> CUCUCUAAAUAGCAAUAUUUACCUUUGGAGGGAAAAGUUAUCAGGCAUGCACCUGGUAGCUAGUCUUUAAACCAAUAGAUUGCAUCGGUUUAAAAGGCAAGACCGUC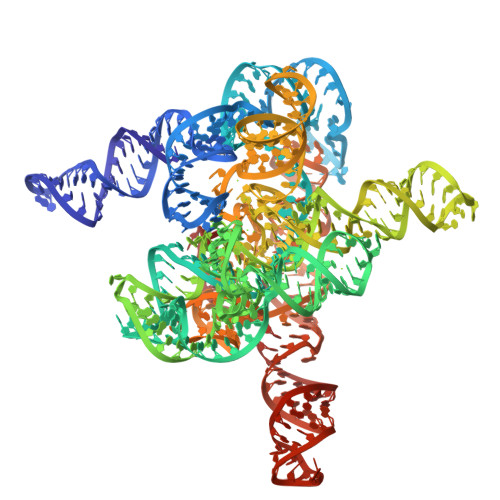AAAUUGCGGGAAAGGGGUCAACAGCCGUUCAGUACCAAGUCUCAGGGGAAACUUUGAGAUGGCCUUGCAAAGGGUAUGGUAAUAAGCUGACGGACAUGGUCCUAACCACGCAGCCAAGUCCUAAGUCAACAGAUCUUCUGUUGAUAUGGAUGCAGUUCACAAACUAAAUGUCGGUCGGGGAAGAUGUAUUCUUCUCAUAAGAUAUAGUCGGACCUCUCCUUAAUGGGAGCUAGCGGAUGAAGUGAUGCAACACUGGAGCCGCUGGGAACUAAUUUGUAUGCGAAAGUAUAUUGAUUAGUUUUGGAGUACUCG> GGTGTGTGGTGGTGTGGTGGTGG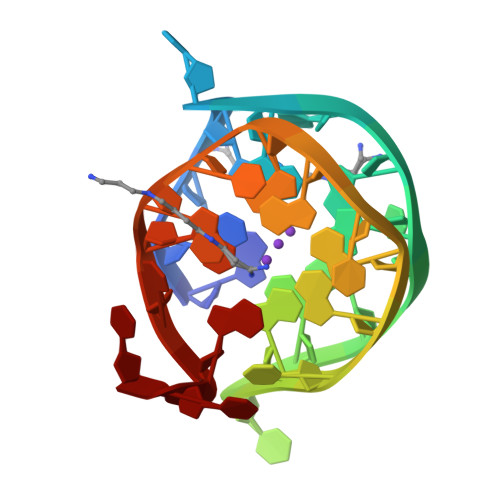TGTT> MTQEFIDKVSSYLTPDVDIAPISQGAEAIVFTTTTHPYLPRAKDSHQKYIIKYRPPKRYRHPQIDQALTKHRTLNESRLLAKLYLIPGLCVPQLIACDPYNGFIWLEFLGEDLPGGHGFSNLKNFLWMHDQDPYSDLVATTLRKVGRQIGLLHWNDYCHGDLTSSNIVLVRDGARWTPHLIDFGLGSVSNLVEDKGVDLYVLERAILSTHSKHAEKYNAWIMEGFEEVYREQGAKGAKKLKEVTKRFEEVRLRGRKRSMLG;> MVVSIIPQFPDIKVSLALFEQVKNAKEIRSKMSELSTSFAFIDPRLV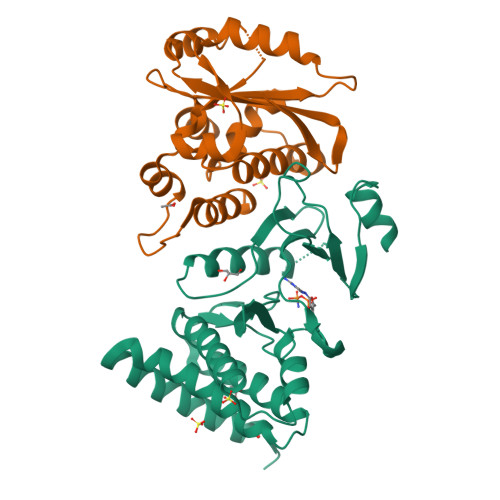CSGEQMYSAIYKTLIEVKYNKMRTRNLNSECVLCLSPTSNISDAFLKFGIKDDSSQLICLKFHTNTDDVDKEQLRTIMTSIVKGQEIEFNDDNLSRFYDEALIRKIYKLSDDFKPQDVNGLSRALVDAIQLRGV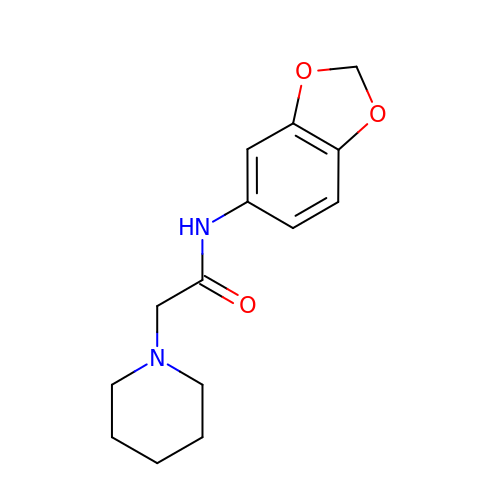N-(1,3-benzodioxol-5-yl)-2-(piperidin-1-yl)acetamide | C14 H18 N2 O3 | KUAQEDPYOBHGFT-UHFFFAOYSA-N> XNVFVGGV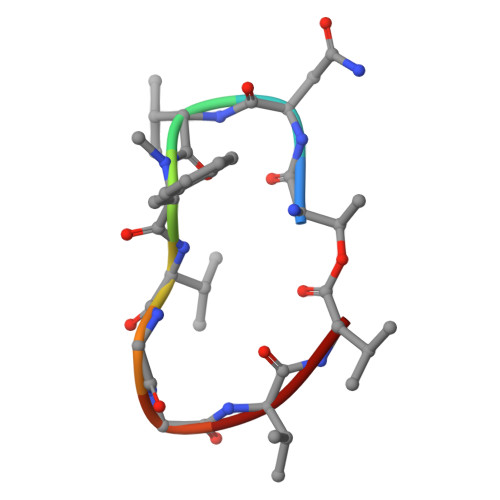L> RITRLQEKEDLQELNDR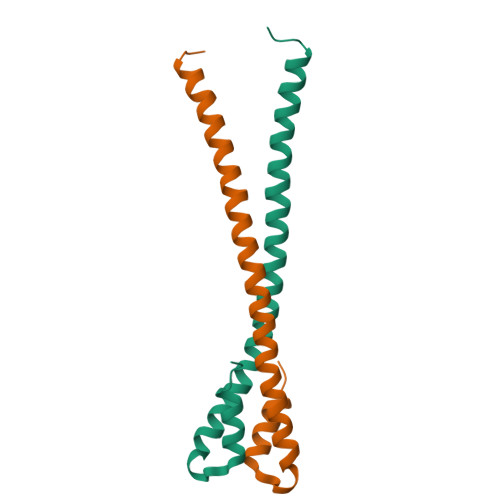LAVYIDRVRSLETENAGLRLRITESEEVVDFYFGKLRNIELICQENEGENDPVLQRIVDILYATDE;> ITRLQEKEDLQELNDRLAVYIDRVRSLETENAGLRLRITESEEVVDFYFGKLRNIELICQENEGENDPVLQRIVDILYATD> MTKSDLLFDKFNDKHGKFLVFFGTFVDTPKLGELRIREKTSVGVLNGIIRFVNRNSLDPVKDCLDHDSSLSPEDVTVVDIIGKDKTRNNSFYFPGFVDTHNHVSQYPNVGVFGNSTLLDWLEKYTFPIEAALANENIAREVYNKVISKTLSHGTTTVAYYNTIDLKSTKLLAQLSSLLGQRVLVGKVCMDTNGPEYYIEDTKTSFESTVKVVKYIRETICDPLVNPIVTPRFAPSCSRELMQQLSKLVKDENIHVQTHLSENKEEIQWVQDLFPECESYTDVYDKYGLLTEKTVLAHCIHLTDAEARVIKQRRCGISHCPISNSSLTSGECRVRWLLDQGIKV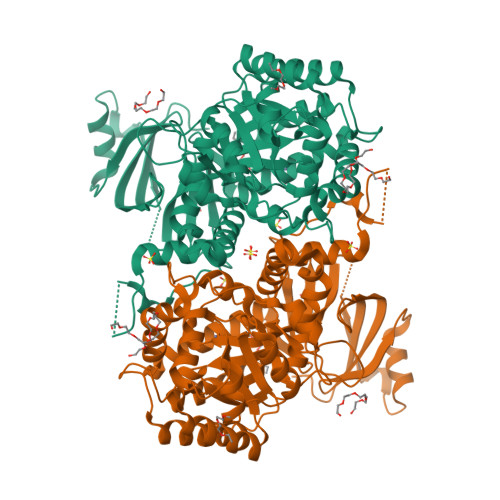GLGTDVSAGHSCSILTTGRQAFAVSRHLAMRETDHAKLSVSECLFLATMGGAQVLRMDETLGTFDVGKQFDAQMIDTNAPGSNVDMFHWQLKEKDQMQEQEQEQGQDPYKNPPLLTNEDIIAKWFFNGDDRNTTKVWVAGQQVYQI>[6x]MKLTPKEQEKFLLYYAGEVARKRKEEGLKLNQPEAIAYISAHIMDEARRGKKTVAQLMEECVHFLKKDEVMPGVGNMVPDLGVEANFPDGTKLVTVNWPIEPDDFKAGEIKFASDKDIELNAGKEITELKVTNKGPKSLHVGSHFHFFEANRALEFDREKAYGKRLDIPSGNTLRIGAGETKTVHLIPIGGSKKIIGMNGLLNGIADDLHKQKALEKAKHHGFIK;>[6x]MKMKRQEYVNTYGPTTGDKVRLGDTDLWAEVEHDYTVYGEELKFGAGKTIREGMGQSNSPDENTLDLVITN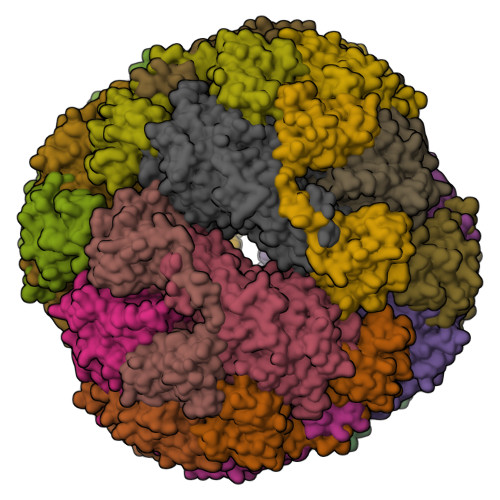ALIIDYTGIYKADIGIKNGKIHGIGKAGNKDMQDGVTPHMVVGVGTEALAGEGMIITAGGIDSHTHFLSPQQFPTALANGVTTMFGGGTGPVDGTNATTITPGVWNLHRMLRAAEEYGMNVGLLGKGNSSSRAQLVEQVKAGAIGFKLHEDWGTTPSAIDHCLSVADEYDVQVCIHTDTVNEAGYVDDTLRAMNGRAIHAYHIEGAGGGHSPDVITMAGEVNILPSSTTPTIPYTINTVAEHLDMLMTCHHLDKRIREDLQFSQSRIRPGSIAAEDTLHDMGVIAMTSSDSQAMGRAGEVIPRTWQTADKNKKEFGRLTEEKGDNDNFRIKRYISKYTINPAITHGVSEYIGSVEEGKIADLVVWNPAFFGVKPKIIIKGGMVVFSEMGDSNASVPTPQPVYYREMFGHHGKAKFDTSITFVSKVAYENGIKEKLGLERKVLPVKNCRNVTKKDFKFNNTTAKITVNPETFEVFVNGKLCTSKPATEVALASRYTFF>MEDLQKALEAQSRALRAELAAGASQSRRPRPPRQRDSSTSGDDSGRDSGGPRRRRGNRGRGQRRDWSRAPPPPEERQETRSQTPAPKPSRAPPQQPQPPRMQTGRGGSAPRPELGPPTNPFQAAVARGLRPPLHDPDTEAPTEACVTSWLWSEG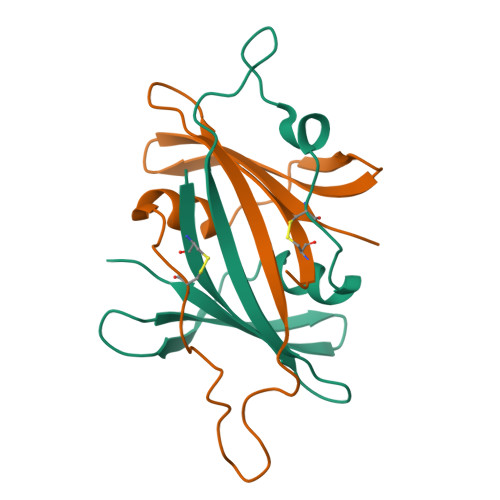EGAVFYRVDLHFTNLGTPPLDEDGRWDPALMYNPCGPEPPAHVVRAYNQPAGDVRGVWGKGERTYAEQDFRVGGTRWHRLLRMPVRGLDGDSAPLPPHTTERIETRSARHPWRIR[2x]>[2x]GSHMGHELAKQEI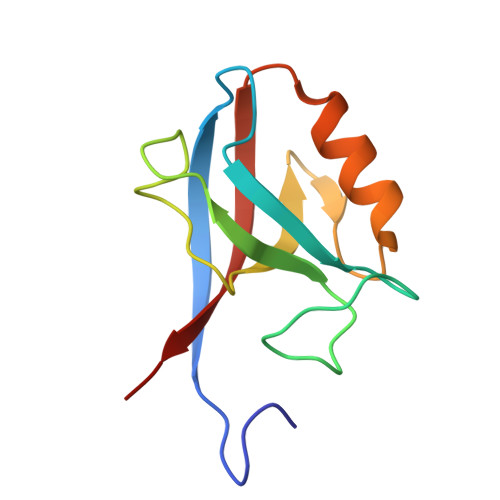RVRVEKDPELGFSISGGVGGRGNPFRPDDDGIFVTRVQPEGPASKLLQPGDKIIQANGYSFINIEHGQAVSLLKTFQNTVELIIVREVSS>ALYEDPPDQKTSPSGKPATLKICSWNVDGLRAWIKKKGLDWVKEEAPDILCLQETKCSENKRPAELQELPGLSHQYWSAPSDKEGYSGVGLLSRQCPLKVSYGIGDEEHDQEGRVIVAEFDSFVLVTAYVPNAGRGLVRLEYRQRWDEAFRKFLKGLASRKPLVLCGDLNVAHEEIDLRNPKGNKKNAG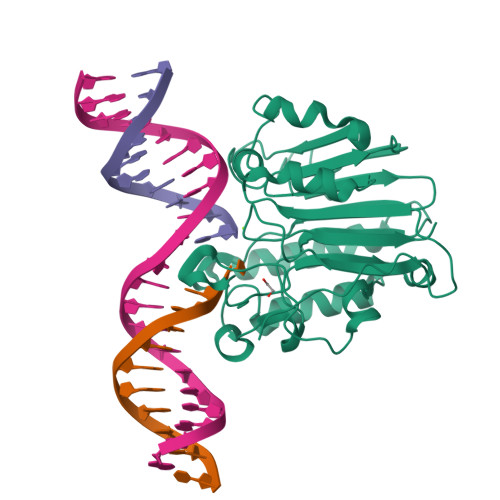FTPQERQGFGELLQAVPLADSFRHLYPNTPYAYTFWTYMMNARSKNVGWRLDYFLLSHSLLPALCDSKIRSKALGSDHCPITLYLAL[2x]>ASNIYKIKEENKNEDICFIAGIGDTNGYGWGIAKELSKRNVKIIFGIWPPVYNIFMKNYKNGKFDNDMIIDKDKKMNILDMLPFDASFDTANDIDEETKNNKRYNMLQNYTIEDVANLIHQKYGKINMLVHSLANAKEVQKDLLNTSRKGYLDALSKSSYSLISLCKYFVNIMKPQSSIISLTYHASQKVVPGYGGGMSSAKAALESDTRVLAYHLGRNYNIRINTISAGPLKSRAATAINKLNNTYENNTNQNKNRNSHDVHNIMNNSGEKEEKKNSASQNYTFIDYAIEYSEKYAPLRQK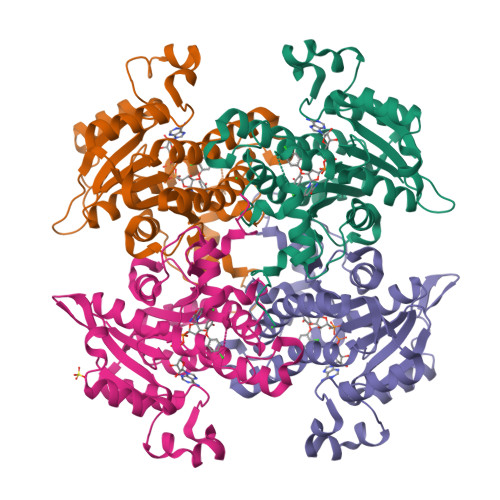LLSTDIGSVASFLLSRESRAITGQTIYVDNGLNIMFLPDDIYRNENE[4x]> MSEPGEEPVAAPAGPAPDPVLNELYGSERPAVELLPGVPLSPIVNSCWLPADAKAMLAESWIPVPPEDAGEEAGPPPPAFEAAAPEYNELVRRLAKTAPFRKWNELTIQAKQLEQEVAGLKGPDAEAKQAELENVKVQIADAEAAVAEVKQSFSDDPLSLTGWMQALTDLADGGMTTFEVSGQGWPYCSLRQLFGEMPSAAPPAGFFDGVERVLGTFKRRYEKERGPGSVQLMLKLAPNVFSDAWSTGGAPAAVAAVEAYVERARANVFGPDGGVTPEGVPEPLDLVQLVWWDFAAADPLPVLKALQRMATDQLQVDEDSGEVSVSEPKKIRGIGLVDFPADRLKAAIQAGVPITCVQVEHSVLVRSAQPVLDLCAKYGIKVLARGGTLGGLLSAKYLGAPPPDPVRGDADLDSVPGCLDAVNNVGGWARLQAALAVIKGIADKHGVKPETVALRWQI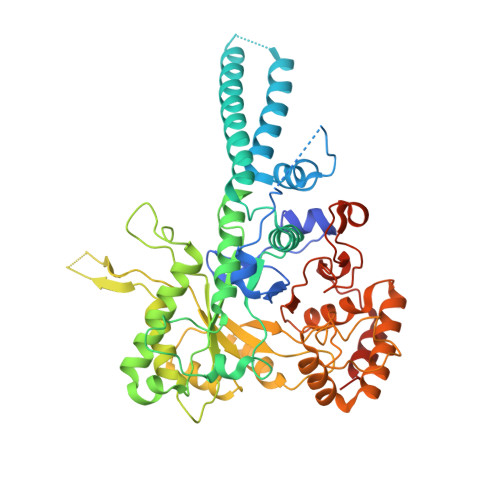DAGCFPLVTTRWSSRVWRQFGYEGWSSFEVSGGRPGVDGPLFQVESFLDVEDVRALAGLAAVHLGPKAG> GSSGSSGMASSCAVQVKLELGHRAQVRKKPTVEGFTHDWMVFVRGPEHSNIQHFVEKVVFHLHESFPRPKRVCKDPPYKVEESGYAGFILPIEVYFKNKEEPRKVRFDYDLFLHLEGHPPVNHLRCEK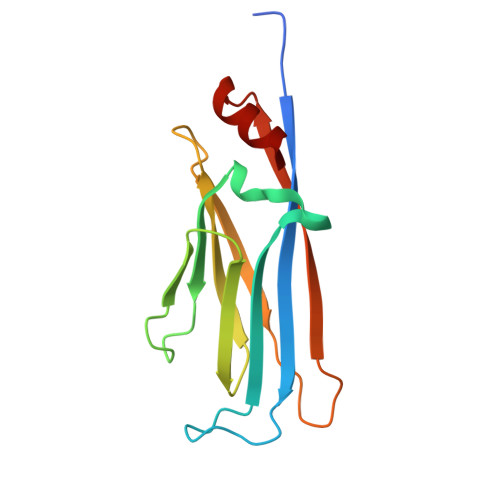LTFNNPTEDFRRKLLKA>MGSHHHHHHDITSLYKKAGSAAAVLEEN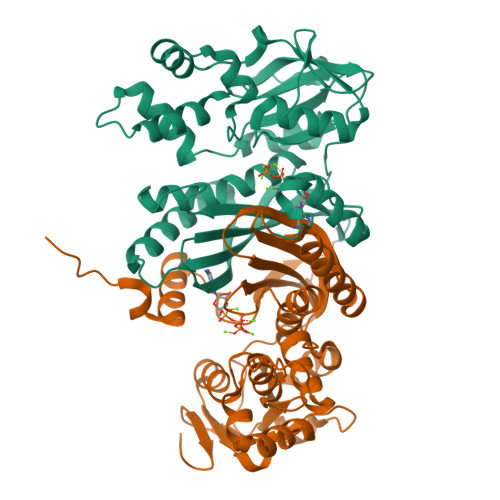LYFQGSFTMRLKELGEFGLIDLIKKTLESKVIGDDTAPVEYCSKKLLLTTDVLNEGVHFLRSYIPEAVGWKAISVNVSDVIANGGLPKWALISLNLPEDLEVSYVERFYIGVKRACEFYKCEVVGGNISKSEKIGISVFLVGETERFVGRDGARLGDSVFVSGTLGDSRAGLELLLMEKEEYEPFELALIQRHLRPTARIDYVKHIQKYANASMDISDGLVADANHLAQRSGVKIEILSEKLPLSNELKMYCEKYGKNPIEYALFGGEDYQLLFTHPKERWNPFLDMTEIGRVEEGEGVFVDGKKVEPKGWKHF[2x]>LDKLHVTSTRPQYVRIKNWGSGEILHDTLHHKATSDFTCKSKSCLGSIMNPKSLTRGPRDKPTPLEELLPHAIEFINQYYGSFKEAKIEEHLARLEAVTKEIETTGTYQLTLDELIFATKMAWRNAPRCIGRIQWSNLQVFDARNCSTAQEMFQHICRHILYATNNGNIRSAITVFPQRSDGKHDFRLWNSQLIRYAGYQMPDGTIRGDAATLEFTQLCIDLGWKPRYGRF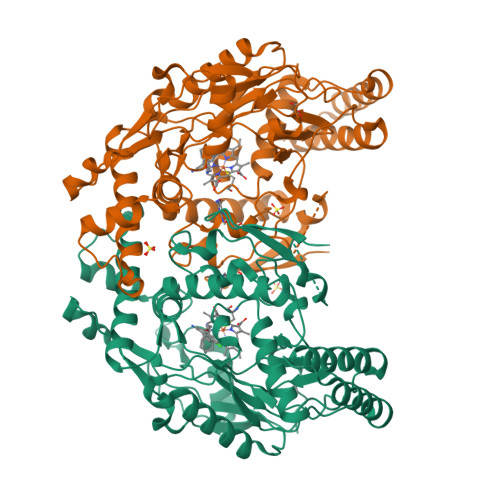DVLPLVLQADGQDPEVFEIPPDLVLEVTMEHPKYEWFQELGLKWYALPAVANMLLEVGGLEFPACPFNGWYMGTEIGVRDFCDTQRYNILEEVGRRMGLETHTLASLWKDRAVTEINVAVLHSFQKQNVTIMDHHTASESFMKHMQNEYRARGGCPADWIWLVPPVSGSITPVFHQEMLNYVLSPFYYYQIEPWKTHIWQNE[2x]>[2x]MAKEEVKQKKTKEKEPDITFFHPDILEVPKDGGLPYLKGYRCKKCGQLDFKTEMCTNCWSEEFEMVPLSRRGKVYSFSDIYIG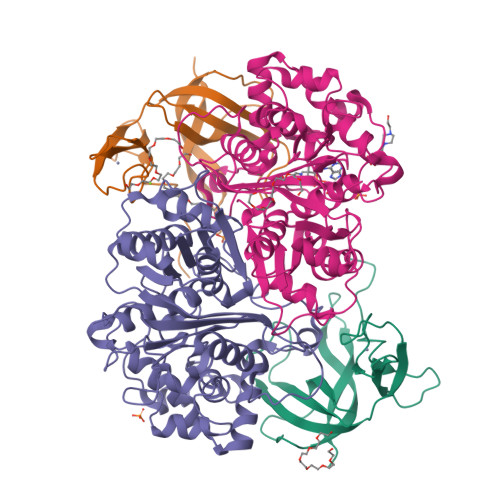QQGLATPYIFAYVDLPENLRVFAQLEGEVDTYRCDEEVELTLGPIRMNNDNLPIISYKFKKIA;>MKLQREVYIAGVGETKFGKHTVDFDVLGREAALQAMNGSNIDRPDMIQSAYVGNGMNDMTTGQAVFRGLGMCGPNLPIINVQSACSAGAMAVFCAIKDVATGVTDLSIGVGTENHTMHRQSGAAFSAARSDIETMHGAVMTGKYAMRATRYMHETGATIEDLAMITVKNRKHATHNPYAWFKGAITVEEVVNSRMVAYPMTLQQCCGIADGAAAVVVGSKEMMKKLGIAKPVKVAGVVVESGPYHNRPRDITGDDITETTSEKLYEESGIGPKEVNILELHDAFTIAELLYYECMGLCKKGDGLKFLRDGQSTYGGQCVVSPRGGLLSYGHPIGASGAAQIAQNVKQLRGECGGYQVGPTPKVAMSHVTGGGLSGTEHAACTMHMLVKGWGS[2x]>GPGSMTDHTRAQVAALVDHTLLKPEATPSDVTALVDEAADLGVFAVCVSPPLVSVAAGVAPSGLAIAAVAGFPSGKHVPGIKATEAELAVAAGATEIDMVIDVGAALAGDLDAVSADITAVRKAVRAATLKVIVESAALLEFSGEPLLADVCRVARDAGADFVKTSTGFHPSGGA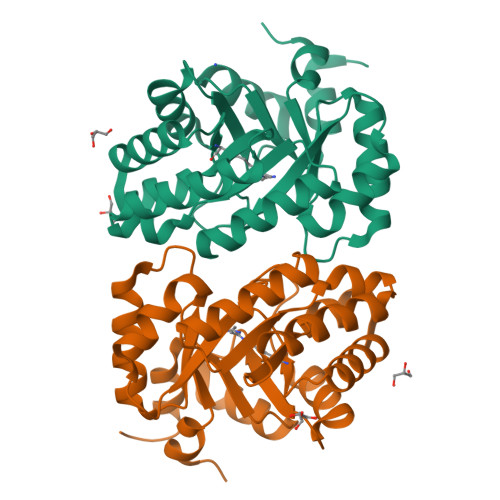SVQAVEIMARTVGERLGVKASGGIRTAEQAAAMLDAGATRLGLSGSRAVLDGFGSA[2x]To explore the outcome of combined exposure to chemicals and establish a detailed mechanistic understanding of this emerging paradigm for EDC action, we focused our attention on the xenoreceptor PXR (pregnane X receptor; NR1I2) which has been identified by the US Environmental Protection Agency ToxCast's program as a major front-line target of chemicals. This NR is a key regulator of the body's defense against foreign substances. It forms heterodimers with the retinoid X receptor (RXR) and binds to PXR responsive elements (PXRE) in the regulatory regions of target genes. To gain structure-based insight into the binding mode of EE2 and TNC to PXR, we solved the crystal structures of PXR-LBD in complex with EE2, TNC, or both at 2.00 Å, 2.55 Å, and 2.25 Å resolution, respectively.

In all cases, the PXR-LBD adopts the canonical active conformation, with the C-terminal activation helix H12 capping the LBP. Whereas EE2 could be precisely placed in the electron densities obtained for both the PXR–EE2 and PXR–TNC–EE2 complexes, TNC could be positioned unambiguously in the ternary complex only. EE2 binds closely adjacent to H12 with a binding mode that is reminiscent of that seen for 17β-estradiol20, both in presence or absence of TNC. The 3-hydroxyl group on the A-ring of EE2 forms an hydrogen bond with S247 (helix H3), whereas the 17β-hydroxyl group on the D-ring is hydrogen bonded with R410 in helix H11 and the main chain oxygen atom of D205 from helix H2'. The position of R410 is further stabilized by a network of hydrogen bonds involving S208 (helix H2') and E321 from the loop preceding H7. The remaining contacts between EE2 and the protein involve van der Waals interactions with several hydrophobic residues. The particular position of EE2 in a restricted region of PXR LBP leaves a significant portion of the pocket unoccupied and available for additional interactions. TNC bound to PXR in a 1:1 molar ratio, while EE2 was found to interact with the receptor with 1:1 and 1:2 binding stoichiometries. Our study shows that individually, EE2 and TNC are too small to make all the necessary interactions ensuring high binding affinity and effective stabilization of the active conformation of the receptor.

> MKKGHHHHHHGSERTGTQPLGVQGLTEEQRMMIRELMDAQMKTFDTTFSHFKNFRLPGVLSSGCELPESLQAPSREEAAKWSQVRKDLCSLKVSLQLRGEDGSVWNYKPPADSGGKEIFSLLPHMADMSTYMFKGIISFAKVISYFRDLPIEDQISLLKGAAFELCQLRFNTVFNAETGTWECGRLSYCLEDTAGGFQQLLLEPMLKFHYMLKKLQLHEEEYVLMQAISLFSPDRPGVLQHRVVDQLQEQFAITLKSYIECNRPQPAHRFLFLKIMAMLTELRSINAQHTQRLLRIQDIHPFATPLMQELFGITGS> MKVLWAALLVTFLAGCQAKVEQAVETEPEPELRQQTEWQSGQRWELALGRFWDYLRWVQTLSEQVQEELLSSQVTQELRALMDETMKELKAYKSELEEQL;> TPVAEETRARLSKELQAAQARLGADMEDVCGRLVQYRGEVQAMLGQSTEELRVRLAS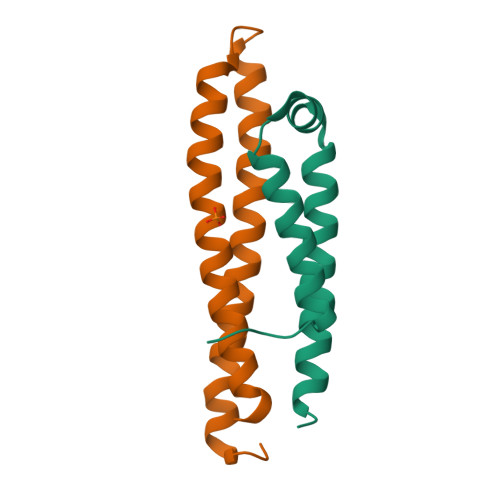HLRKLRKRLLRDADDLQKRLAVYQAG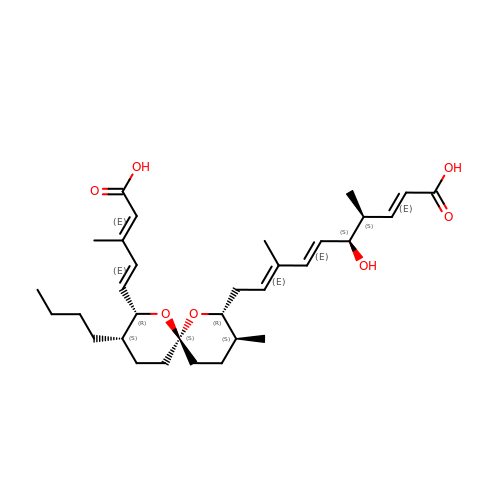(2E,4S,5S,6E,8E)-10-{(2R,3S,6S,8R,9S)-9-butyl-8-[(1E,3E)-4-carboxy-3-methylbuta-1,3-dien-1-yl]-3-methyl-1,7-dioxaspiro[5.5]undec-2-yl}-5-hydroxy-4,8-dimethyldeca-2,6,8-trienoic acid | C32 H48 O7 | YEZCSKCHOPBNCC-OXNFKLAGSA-N> MTLESIMACCLSEEAKEARRINDEIERQLRRDKRDARRELKLLLLGTGESGKSTFIKQMRIIHGSGYSDEDKRGFTKLVYQNIFTAMQAMIRAMDTLKIPYKYEHNKAHA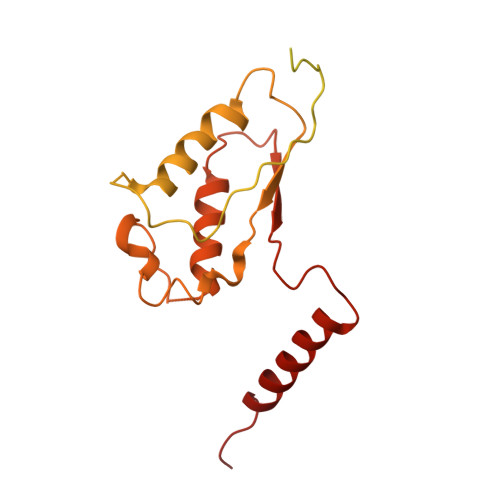QLVREVDVEKVSAFENPYVDAIKSLWNDPGIQECYDRRREYQLSDSTKYYLNDLDRVADPAYLPTQQDVLRVRVPTTGIIEYPFDLQSVIFRMVDVGGQRSERRKWIHCFENVTSIMFLVALSEYDQVLVESDNENRMEESKALFRTIITYPWFQNSSVILFLNKKDLLEEKIMYSHLVDYFPEYDGPQRDAQAAREFILKMFVDLNPDSDKIIYSHFTCATDTENIRFVFAAVKDTILQLNLKEYNLV(2R,3aR,7aR)-2-[(2S)-2-amino-3-hydroxy-3-oxo-propyl]-3,3a,5,6,7,7a-hexahydrofuro[4,5-b]pyran-2-carboxylic acid | C11 H17 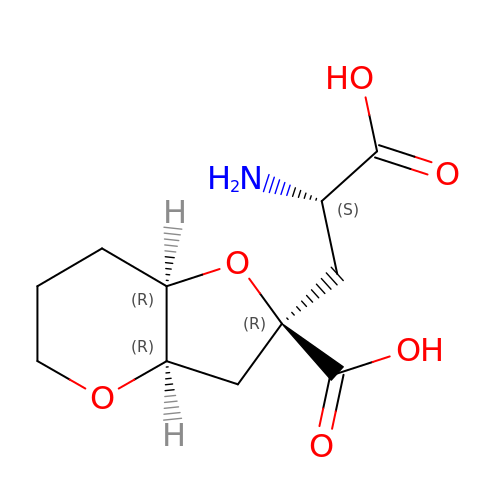N O6 | RZIYCCQNKHONBB-PRKAOEEVSA-N>[4x]MRIPLVGKDSIESKDIGFTLIHEHLRVFSEAVRQQWPHLYNEDEEFRNAVNEVKRAMQFGVKTIVDPTVMGLGRDIRFMEKVVKATGINLVAGTGIYIYIDLPFYFLNRSIDEIADLFIHDIKEGIQGTLNKAGFVKIAADEPGITKDVEKVIRAAAIANKETKVPIITHSNAHNNTGLEQQRILTEEGVDPGKILIGHLGDTDNIDYIKKIADKGSFIGLDRYGLDLFLPVDKRNETTLRLIKDGYSDKIMISHDYCCTIDLGTAKPEYKPKLAPRWSITLIFEDTIPFLKRNGVNEEVIATIFKENPKKFFS

PLLs are natural lactonases endowed with promiscuous phosphotriesterase activity. The catalytic center contained two metal cations coordinated by four histidines, an aspartic acid and a carboxylated lysine residue. A structural analysis of SsoPox, a hyperthermostable counterpart of the PLL family from Sulfolobus solfataricus, has revealed that loop 7 is shorter in SsoPox than in PTEs; linking the active site to the loop 8, which forms a hydrophobic channel that accommodates AHLs aliphatic chain. Indeed, W263 is located at the start of loop 8, involved in the dimer interface of the enzyme and positions the lactone cycle of the substrate onto the bi-metallic catalytic center.

Compared to wild-type SsoPox, variants W263L, W263M and W263F are the most efficient at improving specific activities, ranging from 30-50 and 20-35-fold at 1 mM and 100 µM, respectively. These variants constitute the Phosphotriesterase Selected Variants group (PteSV). Variant W263F is the most proficient (kcat/KM = 1.21 (±0.26)x104 M-1s-1), followed by W263M and W263L with increased efficiencies of 23.3, 14.1 and 4.6-fold, respectively, as compared to wild-type enzyme. Noteworthy, subtle changes, such as W263L or W263I, yield to a large tradeoff in catalytic activities. Regarding the PteSV group, while these variants exhibit higher phosphotriesterase activity, they demonstrate mild improvements for the oxo-lactones and no or wild-type-like AHLase activity (W263L-M and W263F, respectively). Indeed, all variants exhibit a lower Tm compared to the wild-type enzyme (between 92.0 ± 2.1 °C for SsoPox-W263L to 84.1 ± 1.6 °C for SsoPox-W263V). Consequently, substitutions of W263 affect the relative orientation of both monomers; for each mutant, the monomers are closer to each other compared to the wild-type enzyme (with the exception of W263L). The analysis of the normalized B-factors of the variants clearly reveal that the substitution W263 is destabilizing (as confirmed by the Tm of the variants), but also that the active site loops of PteSV are significantly more disordered than those of LacSV. PteSV lose their activity before the loss of the global structure (Tm), whereas LacSV do not, and exhibit a similar thermophilicity profile to that of the wild-type enzyme. These data strongly suggest that the increased disorder in loop 8 caused by the PteSV substitutions collapses the loop as the temperature increase, whereas it does not occur with the LacSV.> M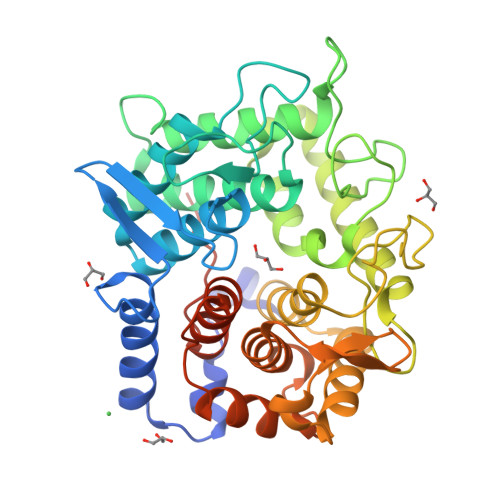EKTTEGAFYTREYRNLFKEFGYSEAEIQERVKDTWEQLFGDNPETKIYYEVGDDLGYLLDTGNLDVRTEGMSYGMMMAVQMDRKDIFDRIWNWTMKNMYMTEGVHAGYFAWSCQPDGTKNSWGPAPDGEEYFALALFFASHRWGDGDEQPFNYSEQARKLLHTCVHNGEGGPGHPMWNRDNKLIKFIPEVEFSDPSFHLPHFYELFSLWANEEDRVFWKEAAEASREYLKIACHPETGLAPEYAYYDGTPNDEKGYGHFFSDSYRVAANIGLDAEWFGGSEWSAEEINKIQAFFADKEPEDYRRYKIDGEPFEEKSLHPVGLIATNAMGSLASVDGPYAKANVDLFWNTPVRTGNRRYYDNCLYLFAMLALSGNFKIWFPEGQEEEHLEHHHHHH> AIYHLTAKTGSRSGGQSARAKADYIQREGKYARDMDEVLHAESGHMPEFVERPADYWDAADLYERANGRLFKEVEFALPVELTLDQQKALASEFAQHLTGAERLPYTLAIHAGGGENPHCHLMISERINDGIERPAAQWFKRYNGKTPEKGGAQKTE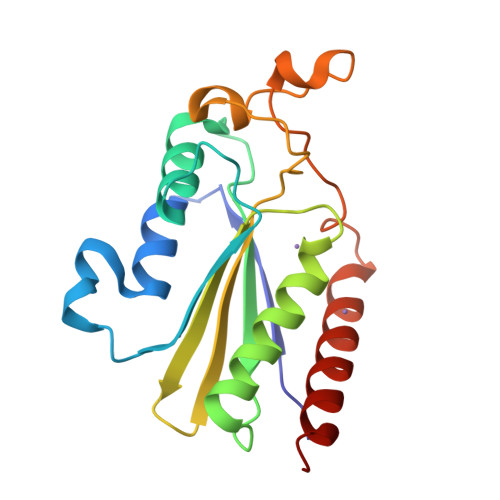ALKPKAWLEQTREAWADHANRALERAGH N-(2,4-dimethoxy-5-{[(2R)-2-methyl-2,3-dihydro-1H-indol-1-yl]sulfonyl}phenyl)acetamide | C19 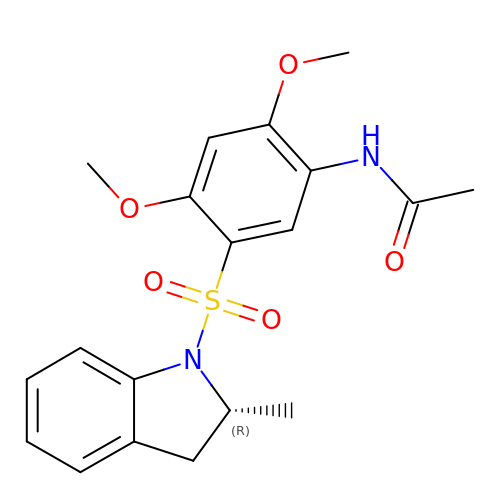H22 N2 O5 S | WCESRWVTCVMYMU-GFCCVEGCSA-N>[2x]MTEHPRAHTAHLRTARLELTPLDPAADARHLHHAYGDEEVMRWWTRPACADPAETERYLTSCAAAPGARLWTIRAPDGTVPGMAGLLGGTDVPGLTWLLRRDSWGHGYATEAAAAVVGHALEDGGLDRVEAWIEAGNRRSLAVAARVGLTERARLAQHYPHRPGPHEMVVLGKARAEEPLTTLAVITELPVRDVAATLRLVEAALGARTAFAIGDPPEFAEAALT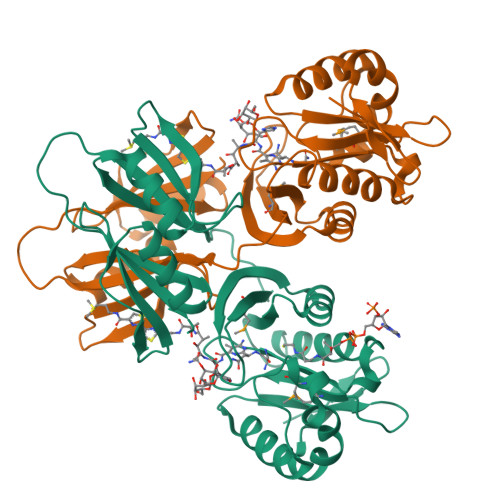PWSAGPRFRLAAVPGPGPVEPVRLHLDAAGTADSLHRRAVDAGARVDGPPVRRPWGRSEFVITLPEGHELTVSAPV Following oxidation of the α-hydroxyl group in GGE by a Cα-dehydrogenase, stereospecific glutathione (GSH)-dependent cleavage of the β-ether linkage in β-(3′-methoxyphenoxy)-γ-hydroxypropiovanillone (MPHPV) is catalyzed by the glutathione S-transferase (GST) enzymes LigE and LigF, forming β-glutathionyl-γ-hydroxypropiovanillone (GS-HPV) and guaiacol. LigE catalyzes stereospecific cleavage of (βR)-MPHPV to (βS)-GS-HPV, whereas LigF catalyzes the cleavage of (βS)-MPHPV to (βR)-GS-HPV. Consistent with their classification as GST enzymes, LigE and LigF each adopt the canonical GST domain fold with an N-terminal thioredoxin domain (residues 1–82 and 1–76, respectively) and a C-terminal α-helical domain (residues 93–255 and 93–242, respectively) connected by a short linker (residues 83–92 and 77–92, respectively). Biochemical and small angle x-ray scattering data suggest that both LigE and LigF exist as dimers in solution, and these dimers, related by 2-fold symmetry, can be seen in the respective crystal structures.

LigFΔ242-GSH crystallized in the space group P6322 with one molecule in the asymmetric unit. Well defined electron density corresponding to the GSH molecule is also visible in the structure. The LigF dimer forms via interactions between helices α3 and α4, in the thioredoxin and C-terminal domains, respectively, of each monomer, forming a four-helix bundle. The dimer interface is largely polar, lacking the traditional lock-and-key motif or hydrophobic surface common in other GST dimers, specifically the Alpha, Pi, and Mu classes. The LigF dimer more closes matches those of the Beta or Theta class, which, like LigF, lack a hydrophobic lock-and-key motif, and there is no open V-shape to the dimer interface. In LigF, Glu-65 and Ser-66 located in the turn connecting β4 and α3, recognize the γ-glutamyl moiety of GSH as part of the ββα motif. Additionally, Gln-52 and the backbone of Val-53 interact with the cysteinyl moiety, whereas Gln-144, His-40, Tyr-148, and Gln-39 anchor the glycine residue of the active site GSH molecule. Due to the occlusion of one face of the GSH binding pocket in LigF, we propose that the substrate binding site is located on the opposite face of the LigF monomer from the dimer interface (black circle). Because LigF Ser-13 was the only potential acid-base catalyst revealed in the active site of the LigFΔ242-GSH structure, we hypothesized that an SN2-type nucleophilic attack mechanism is responsible for catalysis in LigF. Based on our data, LigF is best placed in a new structural class closely related to GSTFuAs or as a fungal Ure2p-like GST based on structural similarities and function in saprotrophic organisms, although it does not strictly fit the class.

> GSHMTLKLYSFGPGANSLKPLATLYEKGLEFEQVFVDPSKFEQHSDWFKKINPRGQVPALWHDGKVVTESTVICEYLEDVFPESGNSLRPADPFKRAEMRVWTKWVDEYFCWCVSTIGWAFGIKAIAQKMSDEEFEEHINKNVPIPEQQLKWRRARNGFPQEMLDEEFRKVGVSVARLEETLSKQDYLVDTGYSLADICNFAIANGLQRPGGFFGDYVNQEKTPGLCAWLDRINARPAIKEMFEKS> SSVSALKRLERSQWTDKMDLRFGFERLKEPGEKTGWLINMHPTEILDEDKRLGSAVDYYFIQDDGSRFKVALPYKPYFYIATRKGCEREVSSFLSKKFQGKIAKVETVPKEDLDLPNHLVGLKRNYIRLSFHTVEDLVKVRKEISPAVKKNREQDHASDAYTALLSSVLQRGGVITDEEETSKKIADQLDNIVDMREYDVPYHIRLSIDLKIHVAHWYNVRYRGNAFPVEITRRDDLVERPDPVVLAFDIETTKLPLKFPDAETDQIMMISYMIDGQGYLITNREIVSEDIEDFEFTPKPEYEGPFCVFNEPDEAHLIQRWFEHVQETKPTIMVTYNGDFFDWPFVEARAAVHGLSMQQEIGFQKDSQGEYKAPQCIHMDCLRWVKRDSYLPVGSHNLKAAAKAKLGYDPVELDPEDMCRMATEQPQTLATYSVSDAVATYYLYMKYVHPFIFALCTIIPMEPDEVLRKGSGTLCEALLMVQAFHANIIFPNKQEQEFNKLTDDGHVLDSETYVGGHVEALESGVFRSDIPCRFRMNPAAFDFLLQRVEKTLRHALEEEEKVPVEQVTNFEEVCDEIKSKLASLKDVPSRIECPLIYHLDVGAMYPNIILTNRLQPSAMVDEATCAACDFNKPGANCQRKMAWQWRGEFMPASRSEYHRIQHQLESEKFPPLFPEGPARAFHELSREEQAKYEKRRLADYCRKAYKKIHITKVEERLTTICQRENSFYVDTVRAFRDRRYEFKGLHKVWKKKLSAAVEVGDAAEVKRCKNMEVLYDSLQLAHKCILNSFYGYVMRKGARWYSMEMAGIVCFTGANIITQARELIEQIGRPLELDTDGIWCVLPNSFPENFVFKTTNVKKPKVTISYPGAMLNIMVKEGFTNDQYQELAEPSSLTYVTRSENSIFFEVDGPYLAMILPASKEEGKKLKKRYAVFNEDGSLAELKGFEVKRRGELQLIKIFQSSVFEAFLKGSTLEEVYGSVAKVADYWLDVLYSKAANMPDSELFELISENRSMSRKLEDYGEQKSTSISTAKRLAEFLGDQMVKDAGLSCRYIISRKPEGSPVTERAIPLAIFQAEPTVRKHFLRKWLKSSSLQDFDIRAILDWDYYIERLGSAIQKIITIPAALQQVKNPVPRVKHPDWLHKKLLEKNDVYKQKKISELFTLEGRRQVTMA;>MFEARLVQGSILKKVLEALKDLINEACWDISSSGVNLQSMDSSHVSLVQLTLRSEGFDTYRCDRNLAMGVNLTSMSKILKCAGNEDIITLRAEDNADTLALVFEAPNQEKVSDYEMKLMDLDVEQLGIPEQEYSCVVKMPSGEFARICRDLSHIGDAVVISCAKDGVKFSASGELGNGNIKLSQTSNVDKEEEAVTIEMNEPVQLTFALRYLNFFTKATPLSSTVTLSMSADVPLVVEYKIADMGHLKYYLAPKIEDEEGS[3x]

Replicative polymerases (Pol), such as the leading-strand polymeraseε (Polε) and lagging-strand Polδ, synthesize DNA with extraordinarily high fidelity. The high accuracy is achieved by their 3′-5′ exonuclease activity, which correct errors when they are made by the DNA polymerase (pol). The POLE1 NTD harbors both DNA polymerase and 3′-5′ proofreading exonuclease (Exo) activities and is therefore referred to as Polε-core in this study. Polε-core interacts with the ring-shaped PCNA sliding clamp to assemble the holoenzyme.

We first asked whether a T/P containing a preexisting mismatch (G•T) can form the expected proofreading intermediates by the Polε–PCNA holoenzyme. Cryo-EM imaging and associated two dimensional (2D) and three dimensional (3D) classifications and 3D reconstruction resulted in two 3D EM maps of the Polε–PCNA–DNA ternary complex at an average resolution of 3.88 Å and 3.81 Å, respectively. Atomic modeling of the two maps shows that Polε-core stably binds to the PCNA and P/T, but the POLE1-CTD and the regulator subunits POLE2-4 are invisible, similar to Polε holoenzyme in the polymerizing state. Notably, the template strand extends to the exo site in both structures, indicating that the T/P with a preexisting mismatch cannot reach the proofreading state in the Polε holoenzyme when the DNA movement is highly constrained by PCNA. Instead, the T/P junction binds just below the Exo and N-term domains in the highly positively charged main substrate chamber, thus placing the holoenzyme in a blocked state. The Exo domain is distant from the thumb in one conformation but interacts with the thumb via a thumb-domain-contacting loop (TCL) in the other conformation. Therefore, the template strand passes through a gap between the TCL and the thumb domain in the first conformation but is blocked by the TCL in the second conformation. While the upper end of the T/P DNA substrate is blocked by Polε, the bottom dsDNA end of the T/P protrudes from PCNA by 6 bp. Remarkably, we found that the tightly coupled PCNA imposes such strong constraints on Polε that a T/P with a preexisting mismatch could not insert from outside of the enzyme into the exo site.>MKMFIGGLSWQTSPDSLRDYFSKFGEIRECMVMRDPTTKRSRGFGFVTFADPASVDKVLGQPHHELDS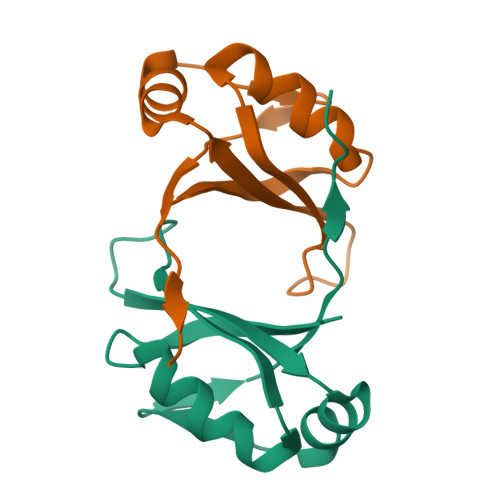KTIDPKVAFPRRAQPK[2x]>[8x]MAETAPLRVQLIAKTDFLAPPDVPWTTDADGGPALVEFAGRACYQSWSKPNPKTATNAGYLRHIMDVGHFSVLEHASVSFYITGISRSCT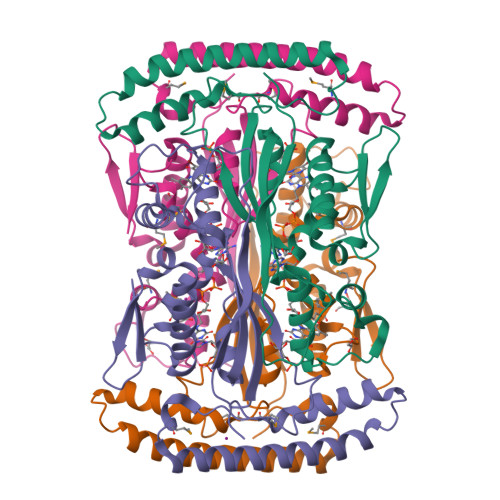HELIRHRHFSYSQLSQRYVPEKDSRVVVPPGMEDDADLRHILTEAADAARATYSELLAKLEAKFADQPNAILRRKQARQAARAVMPNATETRIVVTGNYRAWRHFIAMRASEHADVEIRRLAIECLRQLAAVAPAVFADFEVTTLADGTEVATSPLATEALEHHHHHH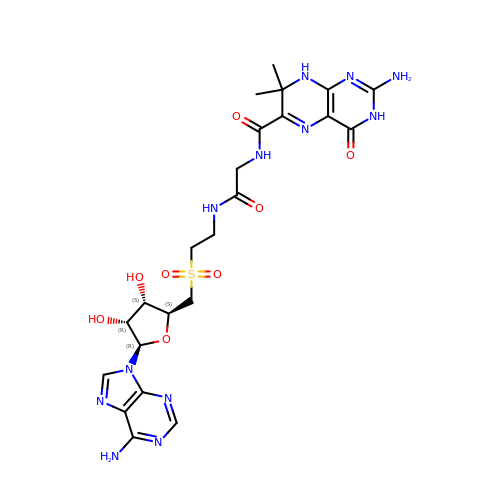5'-{[2-({N-[(2-amino-7,7-dimethyl-4-oxo-3,4,7,8-tetrahydropteridin-6-yl)carbonyl]glycyl}amino)ethyl]sulfonyl}-5'-deoxyadenosine | C23 H30 N12 O8 S | QCWCABDSXQYDST-GWKRVTOESA-N> SAWSHPQFEKENLYFQGTNVRINLDGNTRSFIVPVITTEQIRKNLSYSFYGS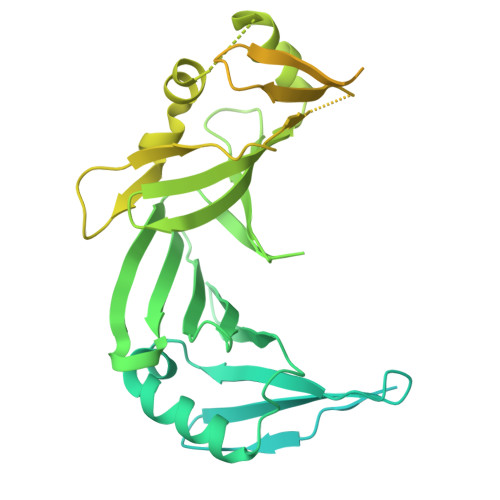GGSYSLSLSPYNMNIDLNLVENDTWVIDVDNVVKNITIESDEIQKGELIENILSKLNIEDNKIVLNNHTINFYGAINESNRFISLTFSILEDINIIIEIDLVSKSYKILLSGNCIKLIENSSDIQQKIDHIGFNGEHQKYIPYSYIDNETKYNGFIDYSKKEGLFTAEFSNESIIRNIYMPDSNNLFIYSSKDLKDIRIINKGDVKLLIGNYFKDNMKVSLSFTIEDTNTIKLNGVYLDENGVAQILKFMNNAKSALNTSNSLMNFLESINIKNIFYNNLDPNIKFILDTNFIISGSNSIGQFELICDKDKNIQPYFIKFKIKETSYTLYAGNRQNLIVEPSYHLDDSGNISSTVINFSQKYLYGIDRYVNKVIITPNLYTDEINITPVYKPNYICPEVIILDANYINEKINININDLSIRYVWDNDGSDLILIANSEEDNQPQVKIRFVNVFKSDTAADKLSFNFSDKQDVSVSKIISTFSLAAGSENLYFQGHHHHHH2-(4-fluorophenoxy)-1-(1H-pyrrol-1-yl)ethan-1-one | C12 H10 F N O2 | 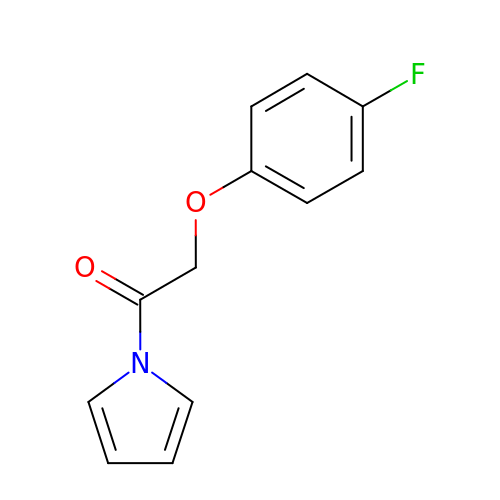ACRFZYHPFRBKAZ-UHFFFAOYSA-N> MASAPIGSAIPRNNWAVTCDSAQSGNECNKAIDGNKDTFWHTFYGANGDPKPPHTYTIDMKTTQNVNGLSVLPRQDGNQNGWIGRHEVYLSSDGTNWGSPVASGSWFADSTTKYSNFETRPARYVRLVAITEANGQPWTSIAEINVFQASSYTAPQP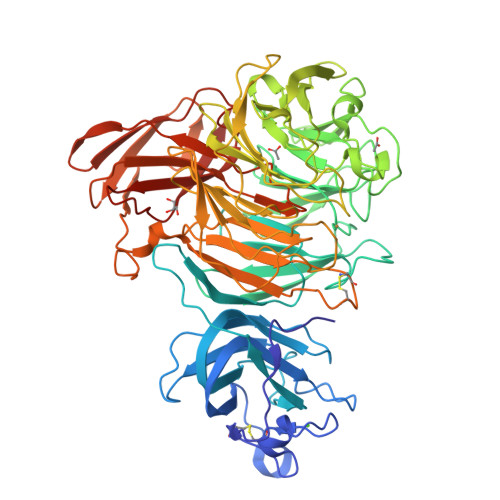GLGRWGPTIDLPIVPAAAAIEPTSGRVLMWSSYRNDAFEGSPGGITLTSSWDPSTGIVSDRTVTVTKHDMFCPGISMDGNGQIVVTGGNDAKKTSLYDSSSDSWIPGPDMQVARGYQSSATMSDGRVFTIGGSWSGGVFEKNGEVYSPSSKTWTSLPNAKVNPMLTADKQGLYRSDNHAWLFGWKKGSVFQAGPSTAMNWYYTSGSGDVKSAGKRQSNRGVAPDAMCGNAVMYDAVKGKILTFGGSPDYQDSDATTNAHIITLGEPGTSPNTVFASNGLYFARTFHTSVVLPDGSTFITGGQRRGIPFEDSTPVFTPEIYVPEQDTFYKQNPNSIVRAYHSISLLLPDGRVFNGGGGLCGDCTTNHFDAQIFTPNYLYDSNGNLATRPKITRTSTQSVKVGGRITISTDSSISKASLIRYGTATHTVNTDQRRIPLTLTNNGGNSYSFQVPSDSGVALPGYWMLFVMNSAGVPSVASTIRVTQLEHHHHHH> TFNPVYP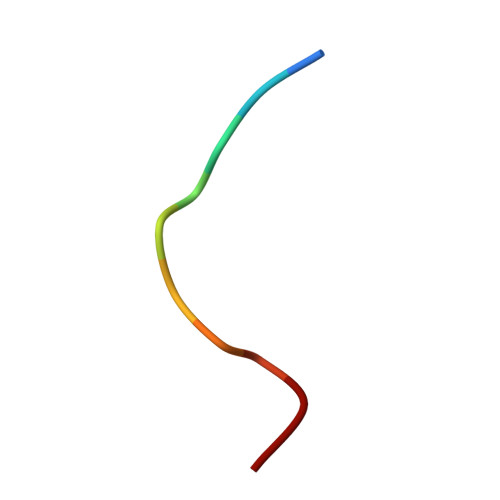YDT> GSMDAKARNCLLQHREALEKDIKTSYIMDHMISDGFLTISEEEKVRNEPTQQQRAAMLIKMILKKDNDSYVSFYNALLHEGYKD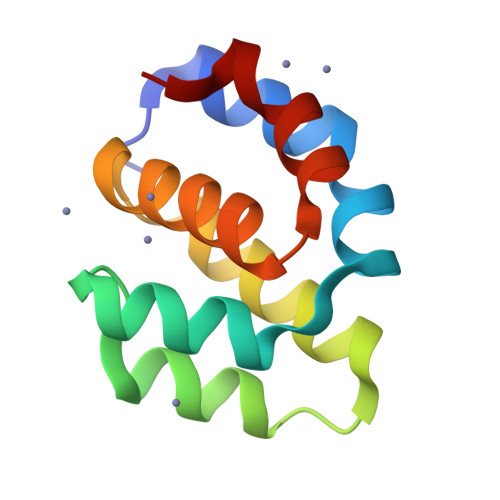LAALLHDGIP> NPVENYIDEVLNEVLVVPNINSSNPTTSNSAPALDAAETGHTSSVQPEDVIETRYVQTSQTRDEMSLESFLGRSGCIHESKLEVTLANYNKENFTVWAINLQEMAQIRRKFELFTYTRFDSEITLVPCISALSQDIGHITMQYMYVPPGAPVPNSRDDYAWQSGTNASVFWQHGQAYPRFSLPFLSVASAYYMFYDGYDEQDQNYGTANTNNMGSLCSRIVT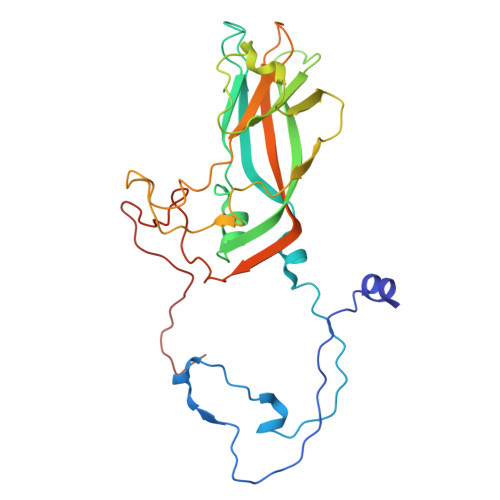EKHIHKVHIMTRIYHKAKHVKAWCPRPPRALEYTRAHRTNFKIEDRSIQTAIVTRPIITTA>[3x]MSKLDTFIQHAVNAVPVSGTSLISSLYGDSLSHRGGEI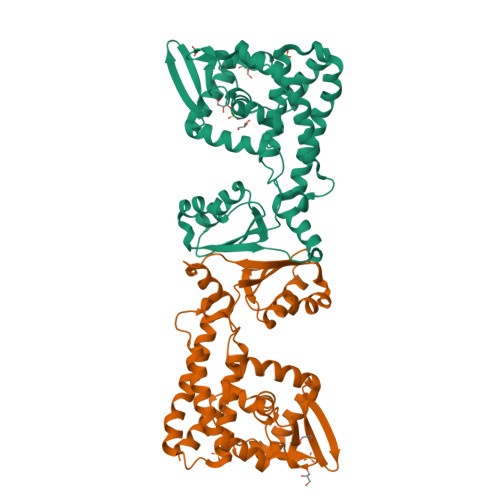WLGSLAALLEGLGFGERFVRTALFRLNKEGWLDVSRIGRRSFYSLSDKGLRLTRRAESKIYRAEQPAWDGKWLLLLSEGLDKSTLADVKKQLIWQGFGALAPSLMASPSQKLADVQTLLHEAGVADNVIAFEAQIPLALSRAALRARVEEAWHLTEQNAMYETFIQSFRPLVPLLKEAADELTPERAFHIQLLLIHFYRRVVLKDPLLPEELLPAHWAGHTARQLAINIYQRVAPAALAFVSEKGETSVGELPAPGSLYFQRFGGLNIEQEALAQFIR> MTW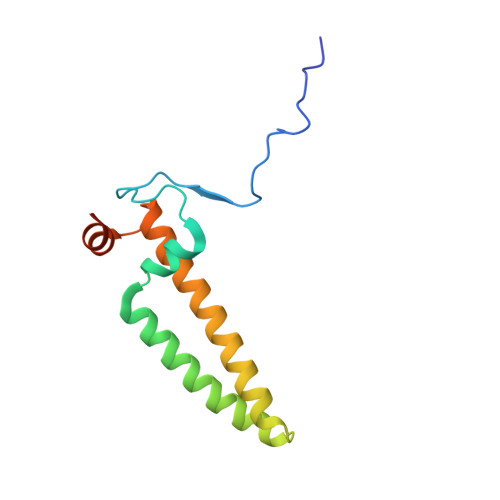PKPINPYDVPSSPAYHRLQEPSYPVIDKDPDFWTAVSNVRKEEWGTTAAVAAGTFVMGYYLGAKGHTGKASAYFTSFLATKSITLYHAYNSADRLMGFKENSREVVKNVPAALVPEHY> NTNDMSPALSAGDGVLYYRLTDRY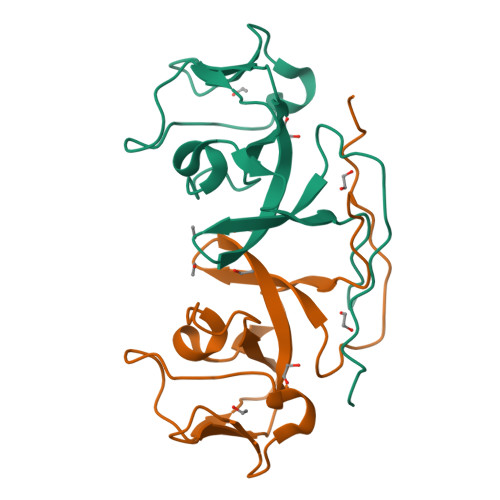HINDVVVYEVDNTLKVGRIAAQAGDEVSFTQEGGLLINGHPPEKEVPYLTYPHSSGPNFPYKVPTGTYFILNDYREERLDSRYYGALPINQIKGKISTLLRVRGI>[2x]GSSGSSGMSVTYDDSVGVEVSSDSFWEVGNYKRTVKRIDDGHR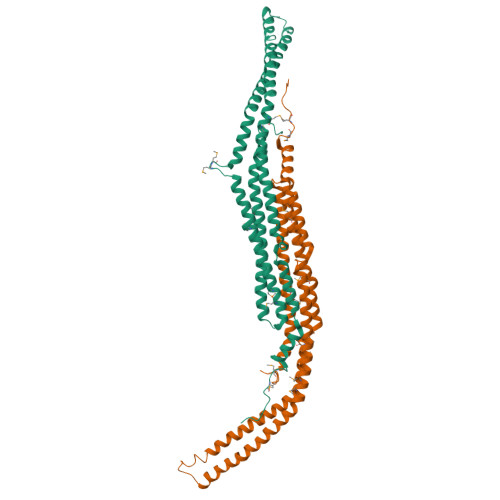LCSDLMNCLHERARIEKAYAQQLTEWARRWRQLVEKGPQYGTVEKAWMAFMSEAERVSELHLEVKASLMNDDFEKIKNWQKEAFHKQMMGGFKETKEAEDGFRKAQKPWAKKLKEVEAAKKAHHAACKEEKLAISREANSKADPSLNPEQLKKLQDKIEKCKQDVLKTKEKYEKSLKELDQGTPQYMENMEQVFEQCQQFEEKRLRFFREVLLEVQKHLDLSNVAGYKAIYHDLEQSIRAADAVEDLRWFRANHGPGMAMNWPQFEEWS> GAMGSWNPKYDTRTLWTTPDTSPNCTIAQDKDSKLTLVLTKCGSQILANVSLIVVAGKYHIINNKTNPKIKSFTIKLLFNKNGVLLDNSNLGKAYWNFRSGNSNVSTAYEKAIGFMPNLVAYPKPSNSKKYARDIVYGTIYLGGKPDQPAVIKTTFNQETGCEYSITFNFSWSKTYENVEFETTSFTFSYIAQE;> MADFARSLSITTPEEMIEKAKGETAYLPCKFTLSPEDQGPLDIEWLISPADNQKVDQVIILYSGDKIYDDYYPDLKGRVHFTSNDLKSGDASINVTNLQLSDIGTYQCKV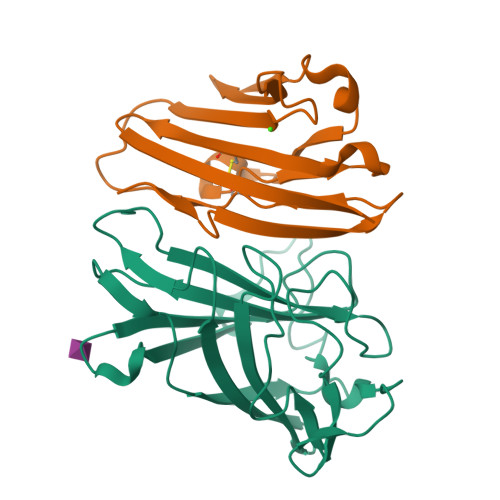KKAPGVANKKIHLVVLGK>PQYQTWEEFSRAAEKLYLADPMKARVVLKYRHSDGNLCVKVTDDLVCLVYKTDQAQDVKKIEKFHSQLMRLMVAKEARNVTMETE[2x];>[2x]VLLESEQFLTELTRLFQKCRTSGSVYITLKKYDGRTKPIPKKGTVEGFEPADNKCLLRATD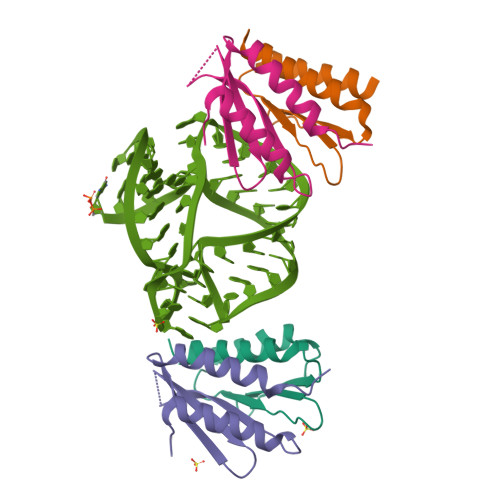GKKKISTVVSSKEVNKFQMAYSNLLRANMDGLKKRDKKNKTKKTK> GPAPNEEFVGDMRIVNVNLSNIDILKKHETFKKYFD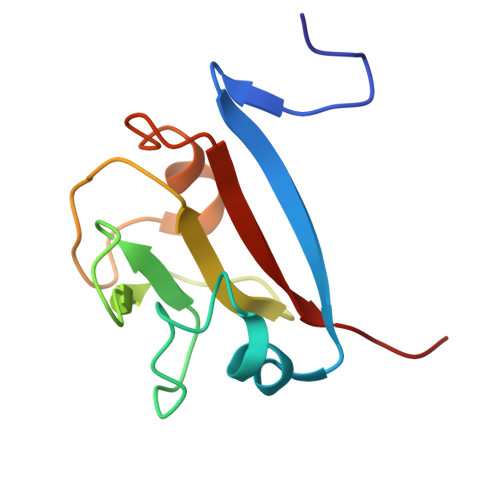FTLTGPRYNGNIAEFAMIWKIKNPPLNLLGVFFDDGTRDDEDDKYILEELKQIGNGAKNMYIFWQYEQK> GGCUUAUCAAGAGAGGUGGAGGGACUGGCCCGAUGAAACCCGGCAACCAGAAAUGGUGCCAAUUCCUGCAGCGGAAACGUUGAAAGAU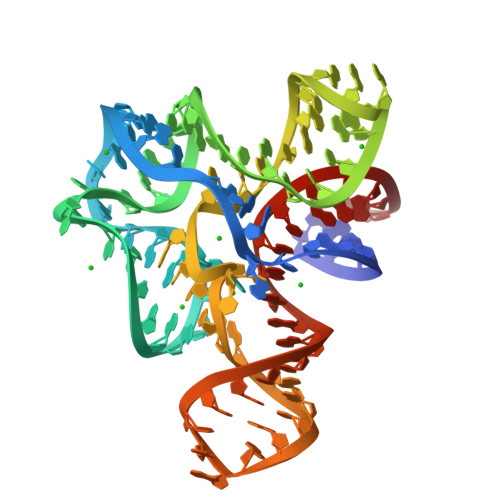GAGCCG> MIEIKDKQLTGLRFIDLFAGLGGFRLALESCGAECVYSNEWDKYAQEVYEMNFGEKPEGDITQVNEKTIPDHDILCAGFPCQAFSIQGKQKGFEDS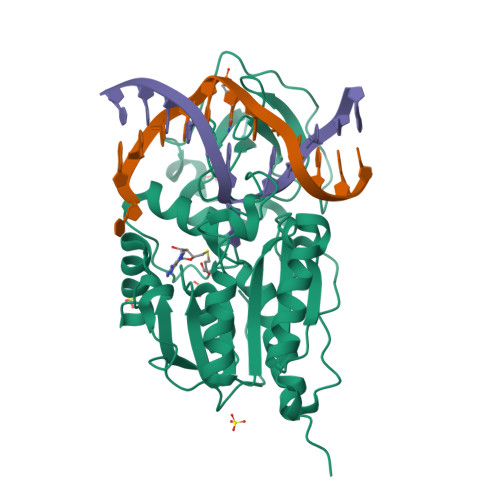RGTLFFDIARIVREKKPKVVFMENVKNFASHDNGNTLEVVKNTMNELDYSFHAKVLNALDYGIPQKRERIYMICFRNDLNIQNFQFPKPFELNTFVKDLLLPDSEVEHLVIDRKDLVMTNQEIEQTTPKTVRLGIVGKGGSGERIYSTRGIAITLSAYGGGIFAKTGGYLVNGKTRKLHPRECARVMGYPDSYKVHPSTSQAYKQFGNSVVINVLQYIAYNIGSSLNFKPY>[12x]MSVNTSFLSPSLV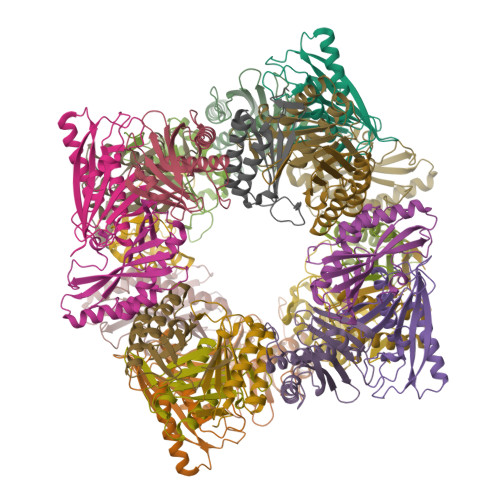TIRDFDKGQFAVLRIGRTGFPADKGDIDLCLSKMDGVLAAQLYLGNPREPGFKGPHIRIRCVDIDDKHTYNAMVYVDLIVGTGASEVERETAEERARRALAVALRVDEADEHSCVTQFEMKLREELLSSDSFHPDKDEYYKDFL;>MPVIQTFVSTPLDHEKRNMLTKVYRIVTDTILGKPAELVMMTFHDSTPMHFFGSTDPVACVRVEALGGYGPSEPEKVTKVVTDAISYVCGIVADRIFVLYFSPLHCGWNGTNLGSHHHHHH[12x]> MEYEWKPDEQGLQQILQLLKESQSPDTTIQRTVQQKLEQLNQYPDFNNYLIFVLTKLKSEDEPTRSLSGLILKNNVKAHFQNFPNGVTDFIKSECLNNIGDSSPLIRATVGILITTIASKGELQNWPDLLPKLCSLLDSEDYNTCEGAFGALQKICEDSAEILDSDVLDRPLNIMIPKFLQFFKHSSPKIRSHAVACVNQFIISRTQALMLHIDSFIENLFALAGDEEPEVRKNVCRALVMLLEVRMDRLLPHMHNIVEYMLQRTQDQDENVALEACEFWLTLAEQPICKDVLVRHLPKLIPVLVNGMKYSDIDIILLKGDVEEDETIPDSEQDIRPRFHRSRTVAQQHDEDGIEEEDDDDDEIDDDDTISDWNLRKCSAAALDVLANVYRDELLPHILPLLKELLFHHEWVVKESGILVLGAIAEGCMQGMIPYLPELIPHLIQCLSDKKALVRSITCWTLSRYAHWVVSQPPDTYLKPLMTELLKRILDSNKRVQEAACSAFATLEEEACTELVPYLAYILDTLVFAFSKYQHKNLLILYDAIGTLADSVGHHLNKPEYIQMLMPPLIQKWNMLKDEDKDLFPLLECLSSVATALQSGFLPYCEPVYQRCVNLVQKTLAQAMLNNAQPDQYEAPDKD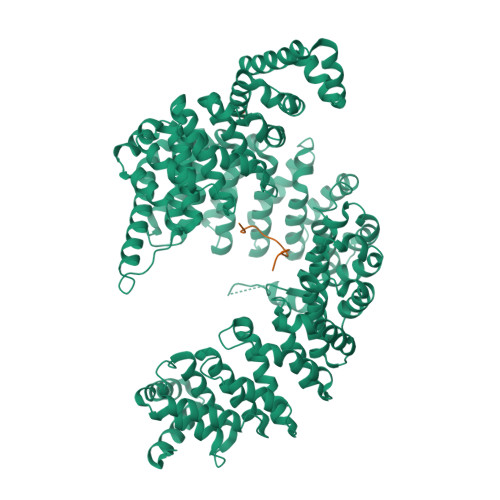FMIVALDLLSGLAEGLGGNIEQLVARSNILTLMYQCMQDKMPEVRQSSFALLGDLTKACFQHVKPCIADFMPILGTNLNPEFISVCNNATWAIGEISIQMGIEMQPYIPMVLHQLVEIINRPNTPKTLLENTAITIGRLGYVCPQEVAPMLQQFIRPWCTSLRNIRDNEEKDSAFRGICTMISVNPSGVIQDFIFFCDAVASWINPKDDLRDMFCKILHGFKNQVGDENWRRFSDQFPLPLKERLAAFYGV;> EEDDGDVAMSDAQDGPRVRYNPYTTRPNRR>SNAFAVSSELSACGRARTYRVEGQLFYGSVEDFMAAFDFREPLERVTIDVSRAHIWDISSVQALDMAVLKFRREGAEVRIVGMNEASE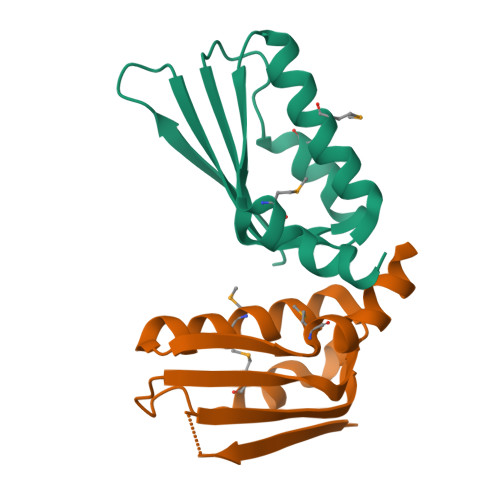TLVDRLALHD[2x]>[2x]MQIVEENLRDNEGEIKLIPETLDDLWHLRFIIEKGDVVFATTKRASQSSDKLRSDKEMVTVRLGIEVEKVEFHRFANRLRVSGKIVAGIEESGYH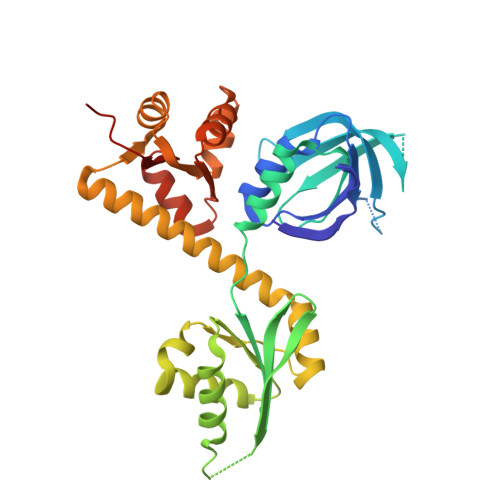TLNITVGKELSIIKKWKPEQLERLRRAVEDSNRPEIVMLTIEEGYAVAGVLRQWGVEEIFEERMGYGKGMGDSRKEFFGEVAAKLESFDFKYLIVAGPGFAKNDFLDFLKERYPEMAKNAVVVDVSSVGSRGFIEILKRRVVDKIVGEVRLAEEAEYIDRLLEGIAKGERVAYGLDEVREAHNYRAIEVLLVADEFLLEEREKWDVDGLLREVEESGGKVVIMSTEFEPGKRLMSLGGIAALLRFNVKGLEHHHHHH>[2x]QSKSRKIAILGYRSVGKSSLTIQFVEGQFVDSADPTIENTFTKLITVNGQEYHL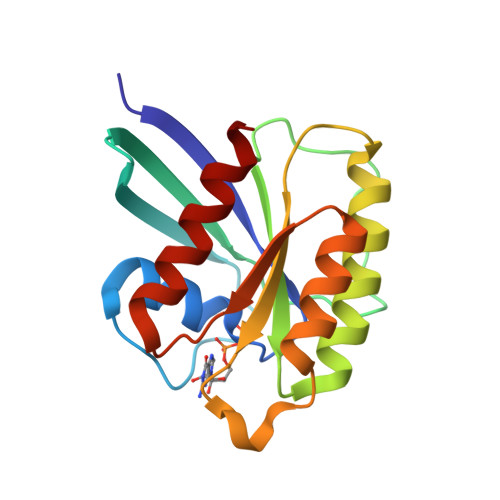QLVDTAGQDEYSIFPQTYSIDINGYILVYSVTSIKSFEVIKVIHGKLLDMVGKVQIPIMLVGNKKDLHMERVISYEEGKALAESWNAAFLESSAKENQTAVDVFRRIILEAEK ACC is then oxidized by the ACC oxidase (ACCO or ACO, referred to as ACO in this study), giving rise to ethylene, carbon dioxide (CO2) and cyanide3. ACO enzyme is a 2OG-oxygenase ‘related' enzyme that belongs to the cupin superfamily, which uses a non-heme ferrous iron (Fe2+) as a cofactor and facilitates the integration of molecular oxygen into a myriad of biomolecules. ACO uses ascorbate, rather than 2-oxoglutarate as the co-substrate, and requires CO2, one of the products of the ACO reaction, as an activator. Overall, the structure of AtACO2 resembles the Petunia hybrid ACO (PhACO), featuring a double-stranded-helix jellyroll fold surrounded by α-helices.

We demonstrate that PZA is also converted to POA in plants, which directly binds to the ACO proteins and inhibits their enzyme activity. In contrast to PZA, POA inhibits the activity of AtACO2 in a concentration dependent manner (IC50=72.05±1.11 μM). POA interacted with AtACO2 in the present of Fe2+, with a dissociation constant (KD) of 14.8 μM. We subsequently co-crystallized AtACO2 with POA or 2-PA in the presence of Zn2+, and determined both structures at 2.1 Å. In both structures, the Zn2+ ion is coordinated by the facial triad, including His180, Asp182 and His237, and binds at a similar position as Fe2+ in PhACO. POA or 2-PA in turn binds to the Zn2+ via the carboxylate group and the N-2 nitrogen in the pyrazine or pyridine ring. The carboxylate group of POA or 2-PA forms a polar interaction with the side chain of Lys161. Besides these polar interactions, the pyrazine/pyridine ring structure also forms hydrophobic/van der Waals interactions with residues including Ile187, Leu189, Ala251 and Phe253. As such, POA or 2-PA would exclude ACC from coordinating with the metal ion, consistent with our kinetic analyses showing that POA is a competitive inhibitor of ACO. The SAR assays revealed the importance of its carboxylic group and the nitrogen in the ortho-position of POA for ACO binding and inhibition, which was validated by the crystal structure of the AtACO2–POA complex.

>MEKNMKFPVVDLSKLNGEERDQTMALINEACENWGFFEIVNHGLPHDLMDKIEKMTKDHYKTCQEQKFNDMLKSKGLDNLETEVEDVDWESTFYVRHLPQSNLNDISDVSDEYRTAMKDFGKRLENLAEDLLDLLCENLGLEKGYLKKVFHGTKGPTFGTKVSNYPPCPKPEMIKGLRAHTDAGGIILLFQDDKVSGLQLLKDGDWIDVPPLNHSIVINLGDQLEVITNGKYKSVLHRVVTQQEGNRMSVASFYNPGSDAEISPATSLVEKDSEYPSFVFDDYMKLYAGVKFQPKEPRFAAMK[2x]> GSHMDVKAEVIEIIDELFMEDVSDMMDEDLFDAGVLDSMGTV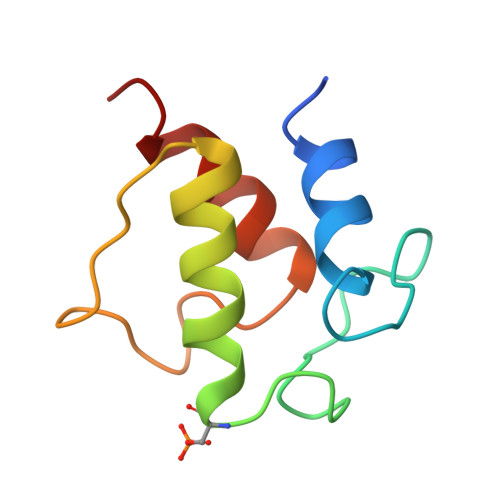ELIVELESRFDIRVPVSEFGRDDWNTANKIVEGVTELRNA> P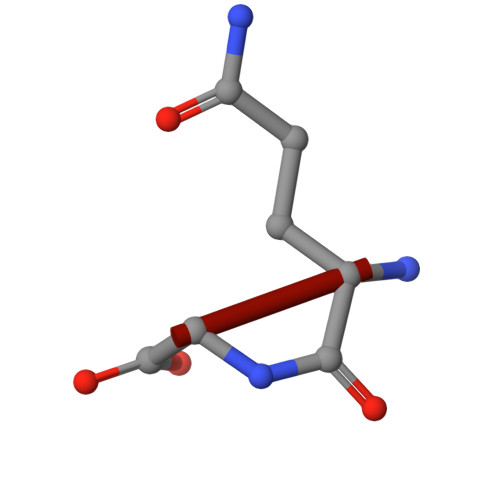QG> MASVHGTTYELLRRQGIDTVFGNPGSNELPFLKDFPEDFRYILALQEACVVGIADGYAQASRKPAFINLHSAAGTGNAMGALSNAWNSHSPLIVTAGQQTRAMIGVEALLTNVDAANLPRPLVKWSYEPASAAEVPHAMSRAIHMASMAPQGPVYLSVPYDDWDKDADPQSHHLFDRHVSSSVRLNDQDLDILVKALNSASNPAIVLGPDVDAANANADCVMLAERLKAPVWVAPSAPRCPFPTRHPCFRGLMPAGIAAISQLLEGHDVVLVIGAPVFRYHQYDPGQYLKPGTRLISVTCDPLEAAR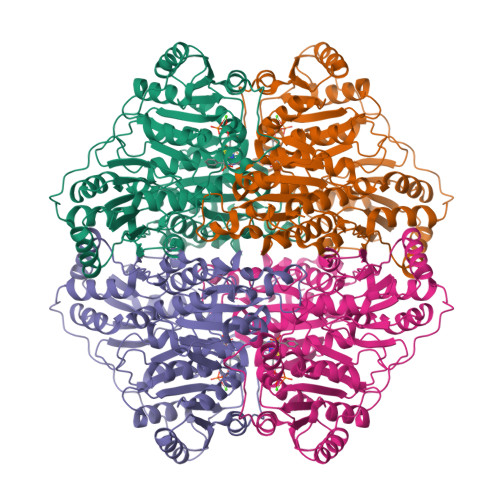APMGDAIVADIGAMASALANLVEESSRQLPTAAPEPAKVDQDAGRLHPETVFDTLNDMAPENAIYLNESTSTTAQMWQRLNMRNPGSYYFCAAGGLGFALPAAIGVQLAEPERQVIAVIGDGSANYSISALWTAAQYNIPTIFVIMNNGTYGALRWFAGVLEAENVPGLDVPGIDFRALAKGYGVQALKADNLEQLKGSLQEALSAKGPVLIEVSTVSPVK The classical model to study retinal proteins is the light-driven proton pump bacteriorhodopsin (bR). Proteins that bind the common biological chromophore retinal are ideal for time-resolved measurements, since they can be activated with a flash of laser light. These proteins fulfil important biological functions, for example, in visual signalling as G-protein-coupled receptors.

Here we present the crystal structure of bR solved by SFX to 2.3 Å resolution using an XFEL. Femtosecond X-ray pulses at XFELs have been demonstrated both theoretically and experimentally to efficiently outrun the radiation damage processes with the exception of highly radiation sensitive metal clusters27. In agreement with this, our bR SFX structure shows no signs of radiation damage in the Asp and Glu residues, where we observed depletion of electron density in our earlier Cryo-structure obtained by conventional crystallography. Intriguingly, the electron density for carboxylic residues is not always better defined when using data from the room temperature measurements SMX and SFX, as compared with the measurements under cryo-conditions. For example, for residue Glu166 the cryo-data gives a very well-resolved electron density for the side chain at 1.5 σ contour level, while the room temperature SMX and SFX structures at this contour level are depleted of density for this residue. In this case, even the protein backbone trace differs between these structures and indicates a mobile region of the protein. The structure obtained at cryogenic temperatures thus seems to favour one conformational state yielding well-defined electron density, albeit a slightly different conformation than for the two room temperature structures. We also observed a small but significant difference within the unconstrained region of the retinal β-ionone ring. These changes can probably be attributed to conformational motions that are obscured at cryogenic temperatures. Difference Fourier maps obtained from a pump-probe experiment with a time delay of 1 ms are compatible with the dark to M state transition and demonstrate the possibility to use an LCP injector for time-resolved crystallography.

> TGRPEWIWLALGTALMGLGTLYFLVKGMGVSDPDAKKFYAITTLVPAIAFTMYLSMLLGYGLTMVPFGGEQNPIYWARYADWLFTTPLLLLDLALLVDADQGTILALVGADGIMIGTGLVGALTKVYSYRFVWWAISTAAMLYILYVLFFGFTSKAESMRPEVASTFKVLRNVTVVLWSAYPVVWLIGSEGAGIVPLNIETLLFMVLDVSAKVGFGLILLRSRAIFG> MSLFKARDWWSTVLGDKEEFDQGCLCLADVDNTGNGQDKIIVGSFMGYLRIFNPHPVKTGDGAQAEDLLLEVHLRDPILQVEVGKFVSGTEMLHLAVLHSRKLCVYSVSGTLGNVEHGNQYQIKLMYEHNLQRTACNMTYGSFGGVKGRDLICIQSVDGMLMVFEQESYAFGRFLPGSLLPGPLAYSSRTDSFITVSSCHQVESYKYQVLAFATDADKRQETEQQKHGSGKRLVVDWTLNIGEQAIDICIVSFIQSASSVFVLGERNFFCLKDNGQIQFMKKLDYSPS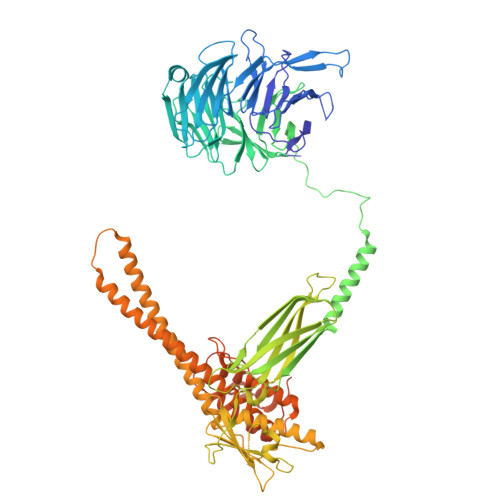CFLPYCSVSEGTINTLIGNHNNMLHIYQDVTLKWATQLPHVPVAVRVGCLHDLKGVIVTLSDDGHLQCSYLGTDPSLFQAPKVESRELNYDELDMELKELQKVIKNVNKSQDVWPLTEREDDLKVSAMVSPNFDSVSQATDVEVGADLVPSVTVKVTLKNRVALQKIKLSIYVQPPLVLTGDQFTFEFMAPEMTRTVGFSVYLKGSYSPPELEGNAVVSYSRPTERNPDGIPRVSQCKFRLPLKLVCLPGQPSKTASHKLTIDTNKSPVSLLSLFPGFAKQSEDDQVNVMGFRFLGGSQVTLLASKTSQRYRIQSEQFEDLWLITNELIIRLQEYFEKQGIKDFTCSFSGSVPLEEYFELIDHHFELRINGEKLEELLSERAVQFRAIQRRLLTRFKDKTPAPLQHLDTLLDGTYKQVIALADAVEENQDNLFQSFTRLKSATHLVILLIGLWQKLSADQIAILEAAFLPLQQDTQELGWEETVDAALSHLLKTCLSKSSKEQALNLNSQLGIPKDTSQLKKHITLFCDRLAKGGRLCLSTDAAAPQTMVMPGGCATIPESDLEGRSIDQDSSELFTNHKHLMVETPVPEVSPLQGVTE> MKTEFSGDTDAVHGKTHVFIRSIKNGSHMQEAKIDIKSLYDSLAKKYDVQHKNSYEVIYPKGYEIKVLGNKYVKLVAMSRHKTQKHLVKIVVKSEKTIDSLDPIRQKSLLKKQDEVVVTTDHICMVYNDDHFFENVNAKNLKVGNYVSVYDEASDKEVIGEIASIEDLGMTDDYVYDCEVDDDSHAFYASNILVHASQFCNGTKLGG

Here, we report the novel and atypically split PolB16 OarG intein and its biochemical and structural characterization. The PolB16 intein carries an atypical split position close to the N-terminal end of the encoded split intein domain to give IntN and IntC fragments of 15 and 168 aa, respectively. Most notably, both residues at the 1 and +1 positions are serine. Furthermore, the intein overall exhibits the typical conserved motifs of a class 1 intein29 that represent conserved residues across inteins, of which some are involved in catalyzing the steps of the protein splicing pathway. This analysis suggested the PolB16 intein splices through linear and branched oxoester intermediates.

To this end, we genetically fused the IntN and IntC precursors, each with 10 extein residues, with a 3 amino acid linker (GSH). Ser1 and Asn183 at the splice junctions were mutated to alanine to block all splicing activity. We obtained protein crystals in this format for both the wild-type sequence and the cysteine-less double mutant (C111A, C165A) and could solve these at resolutions of 1.85 and 2.6 Å, respectively. Both structures were virtually identical (0.185 Å RMSD, root mean square deviation), consistent with the negligible functional impact of mutating the non-conserved cysteine residues (Fig. S6†). No sufficient electron density was found for a part within this region, D86-S95, suggesting it is mobile or less structured, as well as for the termini represented by extein residues (except Asp-1) and the ultimate N183A. The last well-resolved amino acids, Asp108 and His109, show a conformation of the polypeptide chain that departs from the canonical intein structure. As a consequence, His109 is placed in an unusual position, remote from the scissile bond (Fig. 6 and S7C†), which is incompatible with its usual catalytic role. Trying to explain the unusual functional and structural detachment of motif N3:10 residue His109 from the splicing pathway and the intein's active site, we noted in the crystal structures that His68 is positioned in the vicinity of the upstream splice junction.>[4x]GPLGSSAPSV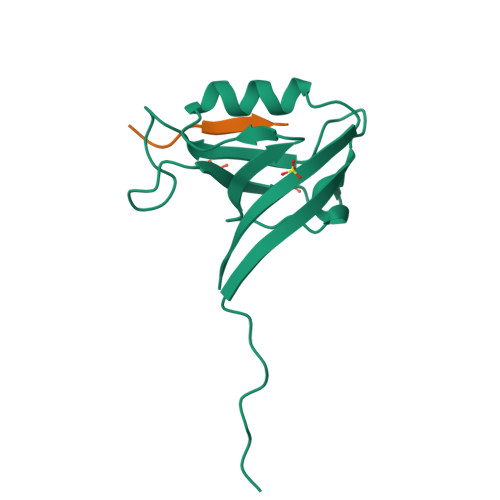KGVSFDQANNLLIEPARIEEEELTLTILRQTGGLGISIAGGKGSTPYKGDDEGIFISRVSEEGPAARAGVRVGDKLLEVNGVALQGAEHHEAVEALRGAGTAVQMRVWRERM;>PAWDETNL[4x]> ASPNSPKDNTWIQAASLTWLMDMSSLLYQLISTRIPSFASPNGLHMREQTIDSNTGQIQIDNEHRLLRWDRRPPNDIFLNGFIPRVTNQNLSPVEDTHLLNYLRTNSPSIFVSTTRARYNNLGLEITPWTPHSANNNIIYRYEIFAPGGIDINASFSRNHNPFPNEDEITFPGGIRPEFIRSTYEYHNGEIVRIWINPNFINPSTLNDVSGPSNISKVFWHENHSEGNNMDSKGFILDLDYNQDFDMFAPNGEIPNNNLLNNNSLNVIQNSEYQIKNKKDRNIVVTLDSDYGGSPVESYKNFGFENQKWNIKYDSKKNAYKIYNRETPTLLLSWNSNSSNGEQVIRGYTESGSNNQYWTIEKNVNGFYKFRNLSDPS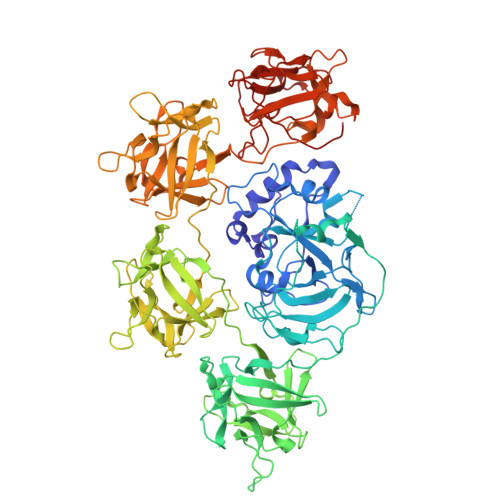KILDLKDGNTLNKTPLVVSSENSSSSQEWLIEKTNYQTVKDGTYQVSSKLNENKVIEQISTNKVHIFSNSDKENQVWNLIYNPILKAYKIKSLKYPNYSLAWDSNNTRTIVAATGDYNDQYWLIERNEDNTYIIRNYENRKIVLDLSNGSTTDGNGLLGFEFHGGINQRWIIKPFSFNSIQDGIYQFMTVINQDLIADLTTNNYTIATKTNNYSSNQKWTVTYNDKKRAYKIRNLQHAHLSLAWDSNHSDKIFGATGDYDDQYWIPILQTDGSFIFRNYKNPNKIFGTNGQPINDIPLKAQDVTGQNNQKWYLRHLNSSNNFTGYFNISSKKNFNKIITMNSNKTQAVIFDNIGINNQSWKLKYNDNKNAYQIHILDNFLYFQGGHNIVATMRNVTNDDLRSYWYVEYNFNKDGFIIRNAFDTSYVLDVFQGNFANNTPIITYQNYLNDNQLWNFIPSLGVEPR In this work, we exhaustively probe the ability of all 36 immobile HJ sequences to form DNA crystals in two different designed systems. Three separate self-assembling DNA crystal systems are described in this report: the “4 × 5” and “4 × 6” designs (collectively referred to as the 4 × N systems), and a third construct with a “scrambled” sequence variant of the 4 × 6 lattices. Self-assembly was mediated by three constituent oligonucleotides: (S1) containing four sequence repeats of either 5 or 6 bases; (S2) composed of 21 bases containing complementary regions to both (S1); and (S3) which forms the second junction crossover. The HJ serves as the fundamental component at the core of each unit, and the ultimate assembly of the full lattice is facilitated by the complementary 2-base sticky ends that tail each duplex.

In parallel, we employed the previously reported J1 4 × 6 system (3.05 Å), with P32 symmetry. Unlike the 4 × 5 motif, nearly all of the 4 × 6 junction sequences had a strong preference for crystallization in buffers containing ≥2.0 M salts (e.g., LiCl, Li2SO4, KCl, and NaCl), with the majority preferring slightly basic pH conditions in cacodylic acid. The average cell constants for the P32 crystals were a = b = 68.29 Å c = 55.68 Å. The c-axis, in particular, was ~5 Å shorter, and had a much larger degree of variability (σ = 1.97), than those that crystallized using the 4 × 5 motif. We show that J1 (or any other junction) should not be considered a privileged option for designing self-assembled lattices. However, in the majority of the crystal structures reported here, the cacodylate anion indeed fits best into the electron density map of our X-ray structures, due to the presence of sodium cacodylate in the crystallization solution.

> GAGCAGACCTGA;> CGGAACTCA;> TCACCG;> TCTGAGTTGGTCTGC> MERIVIVGGGLAASRTCEQLRSRGYEGELVMLCAEPHPPYDRPPLSKAALLEEEHDSTFPTDYAQLSVDVRLGVAATGLVPDARTVQTTDGELSYDALVIATGASPIRLPGPGRQFTVRTVEDAAQLRAELKPGQRVVLVGASWISAEVATAALRRGCSVTCIEAGPAPLSAALGADVGQRFLPWWSEVDLRLDTGVAEVTETGVQLANGEQVDADVVVTGIGVRPAVDWLSGSGIALDTGVVVDEHLRTSLPGIYALGDVAVRWSPRWNTRIRVEHWDDAREAARTLAGVLLHDPSSQDPLPVHDPVPYFWSDQFGHKIQYVGHHSPEDTLVIRGDGTPQWAAAWVDAEGRLTAHLSIDAPRLMIDARMAIAAGARPDEAALRDPQAKLAPP

The ferredoxin reductase FdR9 from Thermobifida fusca, a member of the oxygenase-coupled NADH-dependent ferredoxin reductase (FNR) family, catalyses electron transfer from NADH to its physiological electron acceptor ferredoxin. It forms part of a putative three-component cytochrome P450 monooxygenase system in T. fusca comprising CYP222A1 and the [3Fe–4S]-cluster ferredoxin Fdx8 as well as FdR9. It mediates the transfer of two electrons from NADH to an iron–sulfur cluster-containing ferredoxin via two successive one-electron transfer steps. The overall structure of FdR9 is similar to those of other members of the FNR family and is composed of an FAD-binding domain, an NAD-binding domain and a C-terminal domain.

Here, FdR9 was overexpressed and purified and its crystal structure was determined at 1.9 Å resolution. FdR9 crystallized in space group P4132, with one monomer in the asymmetric unit. The resulting electron-density map allowed the identification of the FAD molecule bound to the reductase. free of 20.0%, displays very good geometry, with no residues located in disallowed regions of the Ramachandran plot. The structure of FdR9 contains nine α-helices and 25 β-strands, which form three distinct domains: an FAD-binding domain (residues 1–106 and 223–308), an NAD-binding domain (residues 107–222) and a C-terminal domain (residues 309–393). The pyrophosphate moiety of FAD is stabilized by hydrogen bonds between the main-chain amide groups of Ala12 and Leu11 and O1P and between the side-chain NH2 group of Arg119 and O2A, as well as between the Asp260 side chain and the O2P and O3′ atoms of the riboflavin part. Moreover, Arg42 plays an important role in stabilizing the FAD cofactor through the formation of electrostatic interactions and hydrogen bonds with the O1A atom of the pyrophosphate moiety and the O3B atom of the adenosine ribose. The first difference involves the presence or absence of secondary structure in the loop region (residues 51–63 in FdR9) of the five ferredoxin reductases. The short and longer helices found in this region in PdR, PuR, ArR and BphA4 correspond to a purely random loop in FdR9. In our FdR9 crystallization experiments we did not attempt to co-crystallize FdR9 with the nicotinamide cofactor, and hence the structure of FdR9 presented here does not contain NAD.> UGCUCCUAGUACGAGAGGACXGGAGU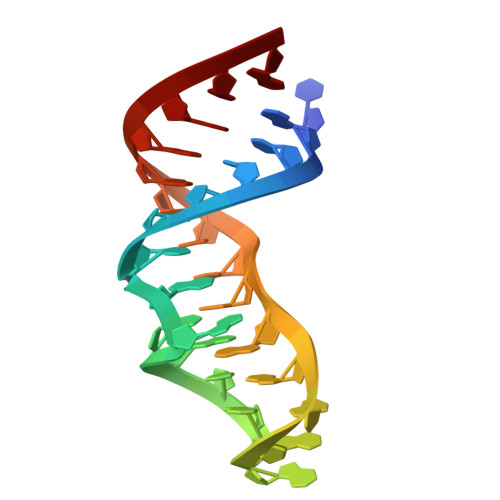G>LTAKHRPSVVWLHNAECTGCTEAAIRTIKPYIDALILDTISLDYQETIMAAAGEAAEAALHQALEGKDGYYLVVEGGLPTIDGGQWGMVAGHPMIETTKKAAAKAKGIICIGTCSAYGGVQKAKPNPSQAKGVSEALGVKTINIPGCPPNPINFVGAVVHVLTKGIPDLDENGRPKLFYGELVHDNCPRLPHFEASEFAPSFDSEEAKKGFCLYELGCKGPVTYNNCPKVLFNQVNWPVQAGHPCLGCSEPDFWDTMTPFYEQG[3x];>MAESKPTPQSTFTGPIVVDPITRIEGHLRIMVEVENGKVKDAWSSSQLFRGLEIILKGRDPRDAQHFTQRACGVCTYVHALASSRCVDDAVKVSIPANARMMRNLVMASQYLHDHLVHFYHLHALDWVDVTAALKADPNKAAKLAASIAPARPGNSAKALKAVQDKLKAFVESGQLGIFTNAYFLGGHKAYYLPPEVDLIATAHYLEALHMQVKAASAMAILGGKNPHTQFTVVGGCSNYQGLTKDPLANYLALSKEVCQFVNECYIPDLLAVAGFYKDWGGIGGTSNYLAFGEFATDDSSPEKHLATSQFPSGVITGRDLGKVDNVDLGAIYEDVKYSWYAPGGDGKHPYDGVTDPKYTKLDDKDHYSWMKAPRYKGKAMEVG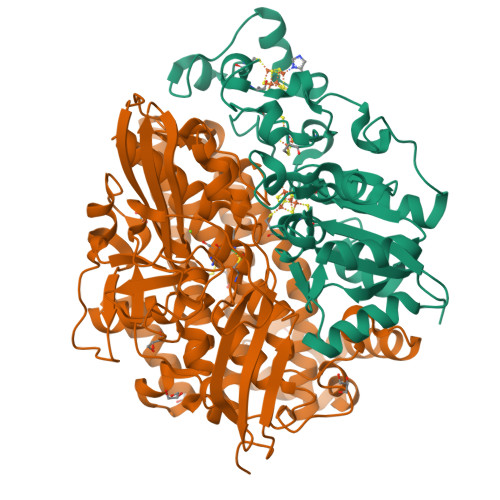PLARTFIAYAKGQPDFKKVVDMVLGKLSVPATALHSTLGRTAARGIETAIVCANMEKWIKEMADSGAKDNTLCAKWEMPEESKGVGLADAPRGALSHWIRIKGKKIDNFQLVVPSTWNLGPRGAQGDKSPVEEALIGTPIADPKRPVEILRTVHAFDPCIACGVH[3x]> KKLIPILEKIPEVELPVKEITFKEKLKWTGIVLVLYFIMGCIDVYTAGAQIPAIFEFWQTITASRIGTLITLGIGPIV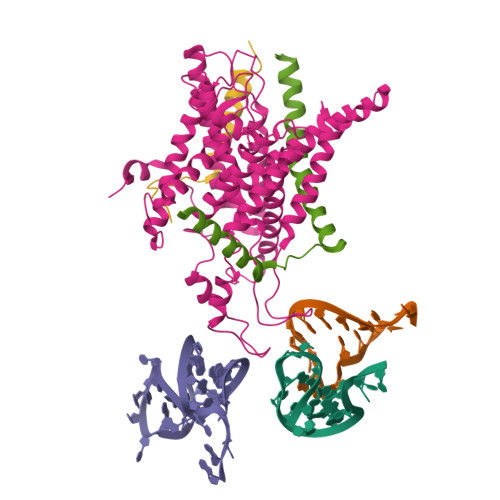TAGIIMQLLVGSGIIQMDLSIPENRALFQGCQKLLSIIMCFVEAVLFVGAGAFGILTPLLAFLVIIQIAFGSIILIYLDEIVSKYGIGSGIGLFIAAGVSQTIFVGALGPEGYLWKFLNSLIQGVPNIEYIAPIIGTIIVFLMVVYAECMRVEIPLAHGRIKGAVGKYPIKFVYVSNIPVILAAALFANIQLWGLALYRMGIPILGHYEGGRAVDGIAYYLSTPYGLSSVISDPIHAIVYMIAMIITCVMFGIFWVETTGLDPKSMAKRIGSLGMAIKGFRKSAIEHRLKRYIPPLTVMSSAFVGFLATIANFIGALGGGTGVLLTVSIVYRMYEQLLREKVSELHPAIAKL;> TDFNQKIEQLKEFIEECRRVWLVLKKPTKDEYLAVAKVTALGISLLGIIGYIIHVPATYIKGILK;> ETFSKIRVKPEHVIGVTVAFVIIEAILTYGRF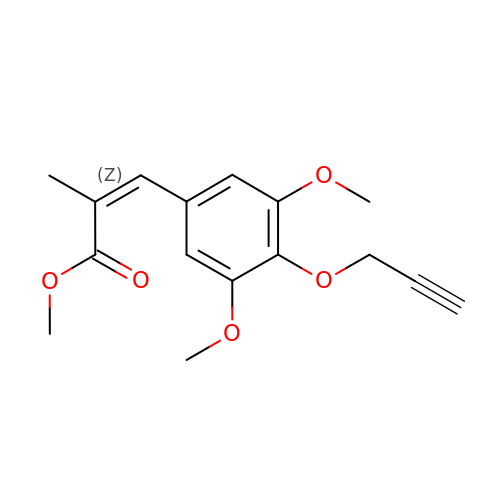methyl (~{Z})-3-(4-ethynoxy-3,5-dimethoxy-phenyl)-2-methyl-prop-2-enoate | C16 H18 O5 | BIIWHDQIRRXQOT-FLIBITNWSA-N>[4x]GHMNRVEPPYDVKEALVFTQKMAQLSKALWKSIEKDWQQWLKP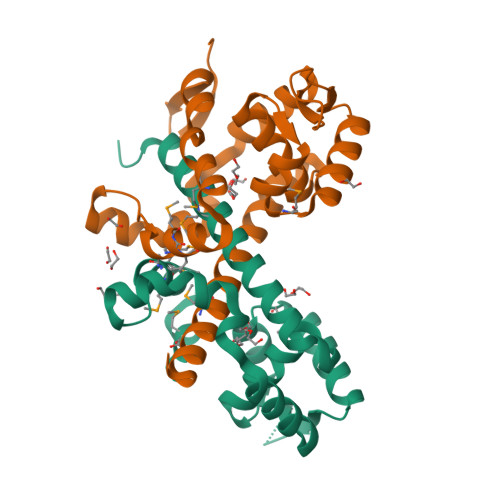YDLNINEHHILWIAYQLNGASISEIAKFGVMHVSTAFNFSKKLEERGYLRFSKRLNDKRNTYVQLTEEGTEVFWSLLEEFDPTRNAVFKGSQPLYHLFGKFPEVAEMMCMIRHIYGDDFMEIFETSLTNIDNDFESVNGKLKKKAKDSAADEPAEELEPVNSGS> GSGHHHHHHGSGDYKDDDDKQDTFTAAVYEHAAILPNATLTPVSREEALALMNRNLDILEGAITSAADQGAHIIVTPEDAIYGWNFNRDSLYPYLEDIPDPEVNWIPCNNRNRFGQTPVQERLSCLAKNNSIYVVANIGDKKPCDTSDPQCPPDGRYQYNTDVVFDSQGKLVARYHKQNLFMGENQFNVPKEPEIVTFNTTFGSFGIFTCFDILFHDPAVTLVKDFHVDTIVFPTAWMNVLPHLSAVEFHSAWAMGMRVNFLASNIHYPSKKMTGSGIYAPNSSRAFHYD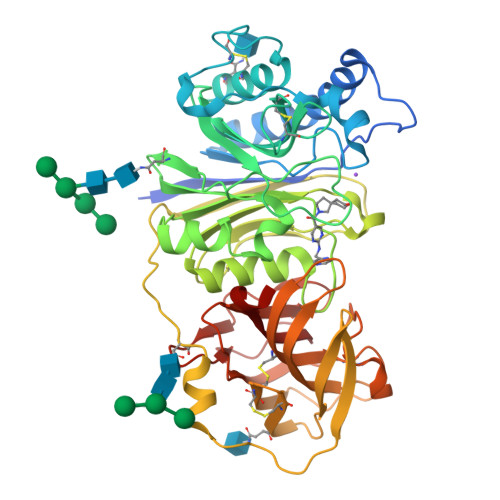MKTEEGKLLLSQLDSHPSHSAVVNWTSYASSIEALSSGNKEFKGTVFFDEFTFVKLTGVAGNYTVCQKDLCCHLSYKMSENIPNEVYALGAFDGLHTVEGRYYLQICTLLKCKTTNLNTCGDSAETASTRFEMFSLSGTFGTQYVFPEVLLSENQLAPGEFQVSTDGRLFSLKPTSGPVLTVTLFGRLYEKD> MELNELTNKLSNLVPMTDFKLDNRASLQLLKYIEAYTKIIPFNSGDKYWNDFFFMSGNTPEKLAKLYQKEIEPNGELLPQQAFLLAVLRLLETPISLLNVLPAAHRELYYRELLGLSSHAAQPDQVALSMELNSTVMEQLLPEGTLFEAGQDEQGNALQYALDASLLANRGYISDLRWLRNDGEKQWVTSAPWDLQAQVSLPSDGIRLFGKTNSDQQVFGGVLITSSLLAMEAGIRKIIVTFEQEMNTQELVAQVSSGNQWLTLTSEVNKKEVTLTLSDKEPAISAPEDLDNLFFTQPVLRLQGKDSQALPEVTGISVSEKDDTKDTSFEMYHLTPFGYSSDIEPLEENPALYLGFTDVKPGQTLALYWKLKSPQQPTVSWYYLDQHNQWAELDSWVSDGTQNLYQDGTWHVELPVDASNQAEQMPVGRYWLRAVVEVPAHEGALGKAPWLYGLIYNAMTATLVNVDSISDSHFLTPLPASSIQRPVEPIIVLASVNQPWASWGGRIPESYSAFFERIAQNLSHRNRSLTWGNMVTLLKERYVSIFDVKYPGNDELTRVPALEQQQLTVIPANRYNDSDDSLRPVLNPARLQEMADWLQQKDSPWASIEVRNPEYLDVKIHYEVIFKPDVNEDFGYRQLQQQLCEVYMPWSIDEQRPVVLNNSINYFQLLATIQQQPLVERVTRLTLHRADSSDESDGTASV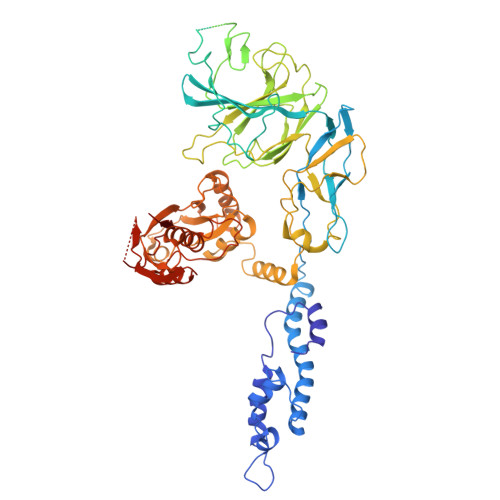EAKDNEVLILVWEEDDNLQYRGNDYE Perforin-2 (MPEG1) is thought to enable the killing of invading microbes engulfed by macrophages and other phagocytes, forming pores in their membranes. Perforin-2 (PFN2) has recently been identified as a novel and critically important component of innate immunity conserved throughout the animal kingdom and evolutionarily close to the last common ancestor of the MAC and perforin-1 (7, 10). Because of the presence of a canonical MAC-perforin (MACPF) domain, PFN2 has been proposed to form functional pores in bacterial membranes, leading to bacterial death and control of infection. However, unlike MAC components and perforin-1, PFN2 is initially synthesized as a type I transmembrane protein and found associated with the membranes of intracellular vesicles in which its large ectodomain (consisting mainly of the MACPF domain and a unique P2 domain characteristic of PFN2) projects into the lumen.

We determined structures of the P2 domain in isolation by x-ray crystallography in two crystal forms, with two crystallographically distinct copies in space group P21 at 2.05 Å and eight copies in space group P1 at 3.17 Å. Truncating the β hairpin (residues Y427-V452) within the P2 domain (P2Δhairpin mutant) abolished its binding to PS, cardiolipin, and E. coli lipids, confirming the role of this region in membrane binding by PFN2. Thus, membrane binding seems to be conferred exclusively by the tip region of the P2 domain β hairpin. The P2 domain helps to stabilize the pre-pore state by swapping between monomers and enables PFN2 to bind its targeted membrane.

>ETGGCTNVDSPNFNFQANMDDDSCDAKVTNFTFGGVYQECTELSGDVLCQNLEQKNLLTGDFSCPPGYSPVHLLSQTHEEGYSRLECKKKCTLKIFCKTVCEDVFRVAKAEFRAYWCVAAGQVPDNSGLLFGGVFTDKTINPMTNAQSCPAGYIPLNLFESLKVCVSLDYELGFKFSVPFGGFFSCIMGNPLVNSDTAKDVRAPSLKKCPGGFSQHLAVISDGCQVSYCVKAGIFTGGSLLPVRLPPYTKPPLMSQVATNTVIVTNSETARSWIKDPQTNQWKLGEGTKHHHHHH[8x]>[2x]TKLEEHLEGIVNIFHQYSVRKGHFDTLSKGELKQLLTKELANTIKNIKDKAVID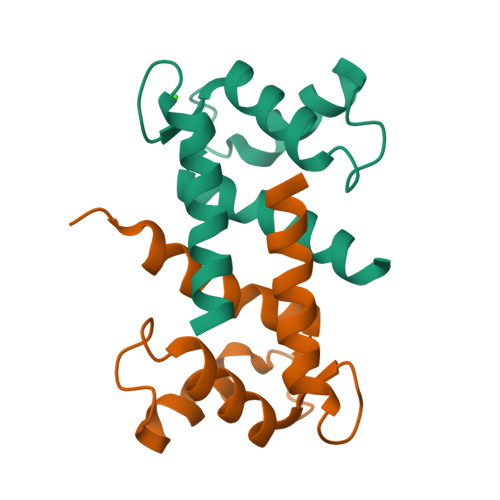EIFQGLDANQDEQVDFQEFISLVAIALKAAHYHTHKE> HHHHHHPVLLRSTDTGQWLRINPDGTVDGTRDRSDPGIQWQISPDGNGPVLLRSTDTGQWLRINPDGTVDGTRDRSDPGIQWQISPDGNGP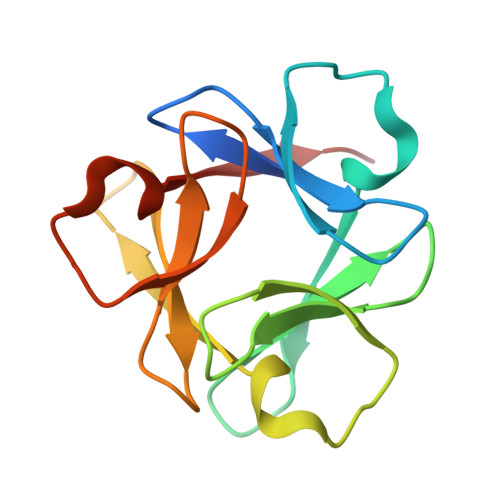VLLRSTDTGQWLRINPDGTVDGTRDRSDPGIQWQISPDGNG(2E)-2-hydroxy-3-(4-hydroxyphenyl)prop-2-enoic 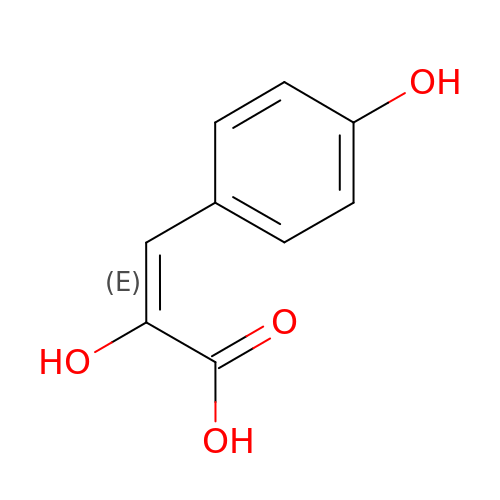acid | C9 H8 O4 | GQYBCIHRWMPOOF-VMPITWQZSA-N The Linker of Nucleoskeleton and Cytoskeleton (LINC) complex crosses both inner and outer nuclear membranes of the nuclear envelope to mechanically transduce cytoskeletal forces to nuclear contents. It is formed of nuclear SUN (Sad1 and UNC84 homology) and cytoplasmic KASH (Klarsicht, ANC-1, and Syne homology) proteins, which interact within the nuclear lumen. JAW1/LRMP (lymphoid restricted membrane protein) is an atypical KASH protein that is localised in the endoplasmic reticulum and outer nuclear membrane, and is specifically expressed in certain cells of the immune system, small intestine, pancreas and taste buds. Here, we report the crystal structure of the SUN-KASH complex between SUN1 and the non-canonical KASH domain of JAW1/LRMP (herein referred to as KASH6).

Thus, we crystallised the SUN1-KASH6 complex and solved its X-ray crystal structures from several crystals at resolutions between 1.7 and 2.3 Å. KASH6 peptides are clearly bound at both of these KASH-binding pockets of each SUN1 trimer (these are herein referred to as KASH6α and KASH6β). The third KASH-binding pocket of each SUN1 trimer is located on the underside of the trimer-of-trimers structure, away from inter-trimer interfaces. In other crystal structures, at resolutions of 2.0 Å and 2.3 Å, we observed no third peptide, with the KASH-binding pocket containing only water molecules. In absence of KASH6γ, the remaining structure was essentially unaltered (r.m.s. deviation = 0.1 Å). Hence, the third binding pocket on the lower surface of the trimer-of-trimers structure cannot stably bind to a KASH6 peptide. We conclude that the SUN1-KASH6 structure is a 9:6 complex in which three SUN1 trimers are bound to six KASH6 peptides. Importantly, the distinct KASH6α and KASH6β conformations result in an asymmetrical structure in which the N-termini of all six KASH6 peptides emanate towards the top surface of the molecule. Hence, uniquely amongst SUN-KASH crystal structures, the SUN1-KASH6 structure is theoretically compatible with outer nuclear membrane insertion.

>[3x]GSGGSGGITEAQARAIVNSALKLYSQDKTGMVDFALESGGGSILSTRCSETYETKTALMSLFGIPLWYFSQSPRVVIQPDIYPGNCWAFKGSQGYLVVRLSMMIHPAAFTLEHIPKTLSPTGNISSAPKDFAVYGLENEYQEEGQLLGQFTYDQDGESLQMFQALKRPDDTAFQIVELRIFSNWGHPEYTCLYRFRVHGEPVK;>GSMEDSWTSLEHILWPFTRLRHNGPPPV[2x]> G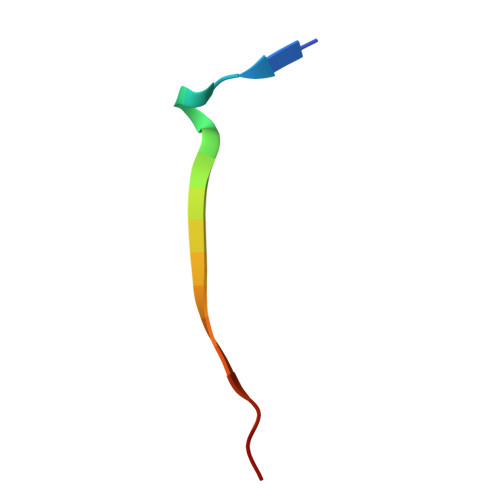SFLPNSEQQKSVDIVFSS>[3x]GTMGVNAVHWFRKGLRLHDNPALKECIQ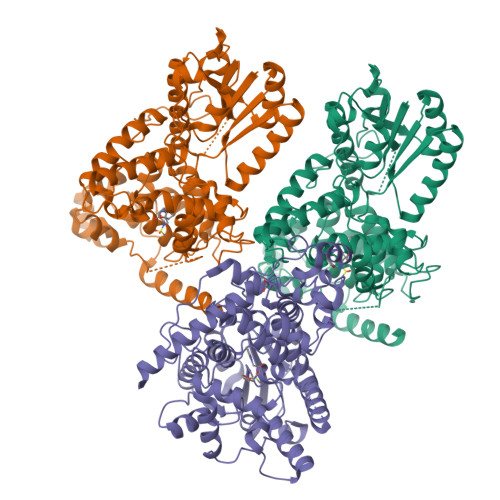GADTIRCVYILDPWFAGSSNVGINRWRFLLQCLEDLDANLRKLNSRLFVIRGQPADVFPRLFKEWNITKLSIEYDSEPFGKERDAAIKKLATEAGVEVIVRISHTLYDLDKIIELNGGQPPLTYKRFQTLVSKMEPLEMPADTITSDVIGKCMTPLSDDHDEKYGVPSLEELGFDTDGLSSAVWPGGETEALTRLERHLERKAWVANFERPRMNANSLLASPTGLSPYLRFGCLSCRLFYFKLTDLYKKVKKNSSPPLSLYGQLLWREFFYTAATNNPRFDKMEGNPICVQIPWDKNPEALAKWAEGRTGFPWIDAIMTQLRQEGWIHHLARHAVACFLTRGDLWISWEEGMKVFEELLLDADWSINAGSWMWLSCSSFFQQFFHCYCPVGFGRRTDPNGDYIRRYLPVLRGFPAKYIYDPWNAPEGIQKVAKCLIGVNYPKPMVNHAEASRLNIERMKQIYQQLSRYRG>[2x]K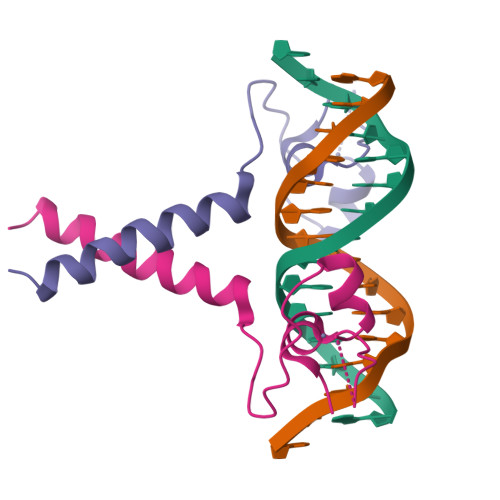RKFACVECRQQKSKCDAHERAPEPCTKCAKKNVPCILKRDFRRTYKRARNEAIEKRFKELTRTLTNLTSDE6-hydroxypyridine-3-carboxylic 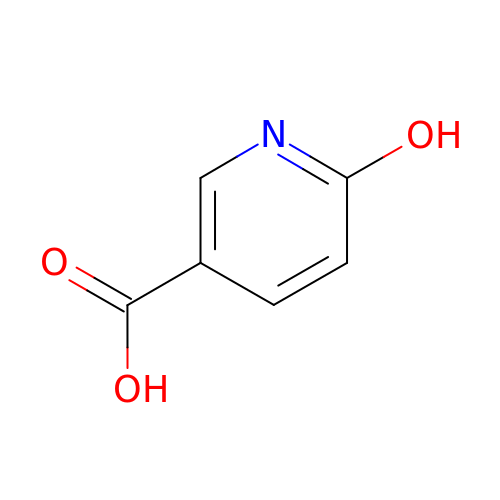acid | C6 H5 N O3 | BLHCMGRVFXRYRN-UHFFFAOYSA-N>[2x]MADVAESQENAPAERAELTVPEMRQWLRNWVGKAVGKAPDSIDESVPMVELGLSSRDAVAMAADIEDLTGVTLSVAVAFAHPTIESLATRIIEGEPETDLAGDDAEDWSRTGPAERVDIAIVGLSTRFPGEMNTPEQTWQALLEGRDGITDLPDGRWSEFLEEPRLAARVAGARTRGGYLKDIKGFDSEFFAVAKTEADNIDPQQRMALELTWEALEHARIPASSLRGQAVGVYIGSSTNDYSFLAVSDPTVAHPYAITGTSSSIIANRVSYFYDFHGPSVTIDTACSSSLVAIHQGVQALRNGEADVVVAGGVNALITPMVTLGFDEIGAVLAPDGRIKSFSADADGYTRSEGGGMLVLKRVDDARRDGDAILAVIAGSAVNHDGRSNGLIAPNQDAQADVLRRAYKDAGIDPRTVDYIEAHGTGTILGDPIEAEALGRVVGRGRPADRPALLGAVKTNVGHLESAAGAASMAKVVLALQHDKLPPSINFAGPSPYIDFDAMRLKMITTPTDWPRYGGYALAGVSSFGFGGANAHVVVREVLPRDVVEKEPEPEPEPKAAAEPAEAPTLAGHALRFDEFGNIITDSAVAEEPEPELPGVTEEALRLKEAALEELAAQEVTAPLVPLAVSAFLTSRKKAAA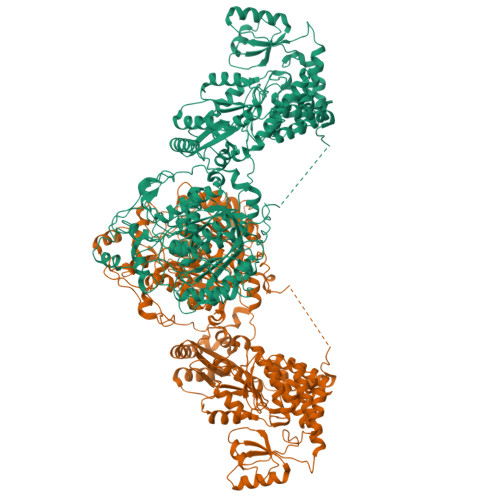AELADWMQSPEGQASSLESIGRSLSRRNHGRSRAVVLAHDHDEAIKGLRAVAAGKQAPNVFSVDGPVTTGPVWVLAGFGAQHRKMGKSLYLRNEVFAAWIEKVDALVQDELGYSVLELILDDAQDYGIETTQVTIFAIQIALGELLRHHGAKPAAVIGQSLGEAASAYFAGGLSLRDATRAICSRSHLMGEGEAMLFGEYIRLMALVEYSADEIREVFSDFPDLEVCVYAAPTQTVIGGPPEQVDAILARAEAEGKFARKFATKGASHTSQMDPLLGELTAELQGIKPTSPTCGIFSTVHEGRYIKPGGEPIHDVEYWKKGLRHSVYFTHGIRNAVDSGHTTFLELAPNPVALMQVALTTADAGLHDAQLIPTLARKQDEVSSMVSTMAQLYVYGHDLDIRTLFSRASGPQDYANIPPTRFKRKEHWLPAHFSGDGSTYMPGTHVALPDGRHVWEYAPRDGNVDLAALVRAAAAHVLPDAQLTAAEQRAVPGDGARLVTTMTRHPGGASVQVHARIDESFTLVYDALVSRAGSESVLPTAVGAATAIAVADGAPVAPETPAEDADAETLSDSLTTRYMPSGMTRWSPDSGETIAERLGLIVGSAMGYEPEDLPWEVPLIELGLDSLMAVRIKNRVEYDFDLPPIQLTAVRDANLYNVEKLIEYAVEHRDEVQQLHEHQKTQTAEEIARAQAELLHGKVGKTEPVDSEAGVALPSPQNGEQPNPTGPALNVDVPPRDAAERVTFATWAIVTGKSPGGIFNELPRLDDEAAAKIAQRLSERAEGPITAEDVLTSSNIEALADKVRTYLEAGQIDGFVRTLRARPEAGGKVPVFVFHPAGGSTVVYEPLLGRLPADTPMYGFERVEGSIEERAQQYVPKLIEMQGDGPYVLVGWSLGGVLAYACAIGLRRLGKDVRFVGLIDAVRAGEEIPQTKEEIRKRWDRYAAFAEKTFNVTIPAIPYEQLEELDDEGQVRFVLDAVSQSGVQIPAGIIEHQRTSYLDNRAIDTAQIQPYDGHVTLYMADRYHDDAIMFEPRYAVRQPDGGWGEYVSDLEVVPIGGEHIQAIDEPIIAKVGEHMSRALGQIEADRTSEVGKQ>MSKLLVVKAHPLTKEESRSVRALETFLASYRETNPSDEIEILDVYAPETNMPEIDEELLSAWGALRAGAAFETLSENQQQKVARFNELTDQFLSADKVVIANPMWNLNVPTRLKAWVDTINVAGKTFQYTAEGPKPLTSGKKALHIQSNGGFYEGKDFASQYIKAIL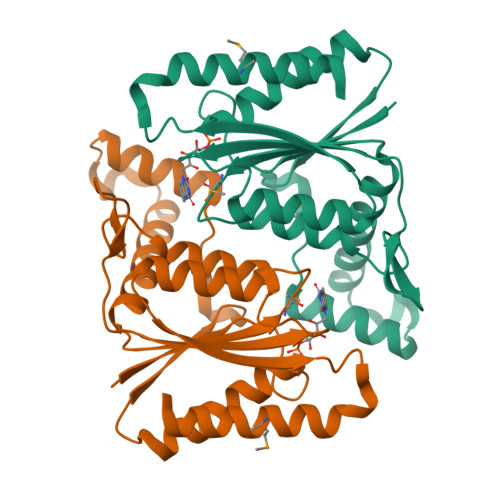NFIGVDQVDGLFIEGIDHFPDRAEELLNTAMTKATEYGKTF[4x]> SNAMIWTTGKTLCKTQKRPRNPYFAQAYDFMEKWLGGAREFVLHTSGSTGMPKPITVTRAQLAASAAMTGKALSLGPGTRALVCLNVGYIAGLMMLVRGMELDWELTVTEPTANPLAGLDHADFDFVAMVPMQLQSILENSATSGQVDRLGKVLLGGAPVNHALAMQISDLAMPVYQSYGMTETVSHVALKALNGPEASELYVFLPGIQYGVDERGCLHISGAVTNGQTVQTNDLVEIHGNAFQWIGRADNVINSGGVKIVLDQIDQRIAAVFHHLNIGNAFFCWWEPDAKLGQKLVLVIENAMPEALTERLTAEIRSRVSTYENPKHIYFAKAFAKTQTD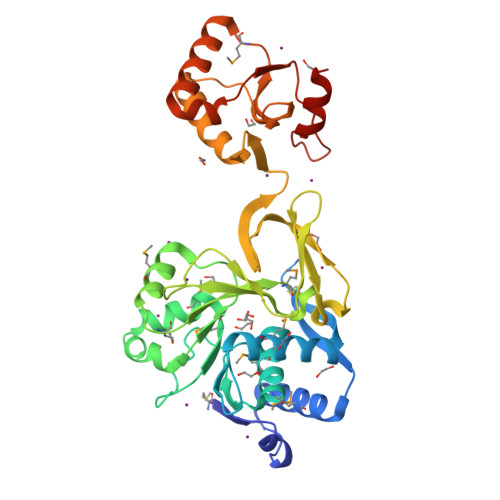KIDKRATFQKLSDSSNG> MSSTPSNQNIIPIIKKESIVSLFEKGIRQDGRKLTDYRPLSITLDYAKKADGSALVKLGTTMVLAGTKLEIDKPYEDTPNQGNLIVNVELLPLAYTTFEPGPPDENAIELARVVDRSLRDSKALDLTKLVIEPGKSVWTVWLDVYVLDYGGNVLDACTLASVAALYNTKVYKVEQISVNKNEVVGKLPLNYPVVTISVAKVDKYLVVDPDLDEESIMDAKISFSYTPDLKIVGIQKSGKGSMSLQDIDQAENTARSTAV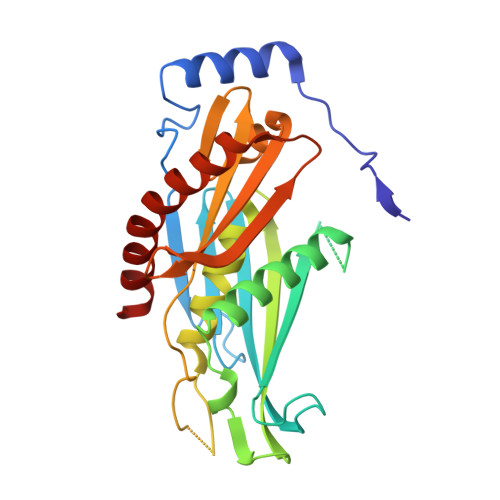KLLEELKKHLGI> KEAIVFSQKTTIDQLHNSLNAASKTGNSNEVLQDPHIGDMYGSVTPLRPQVTRMLGKYAKEKEDMLSLRQVLANAERSYNQLMDRAAN;> VDLSDEEKDSIYMFASLVEKMKSRPLNEILEDSKLQNLAQRVFASKARLNYALNDKAQKYNTLIEMNGKISEIMNIYDRLLEQQLQSINL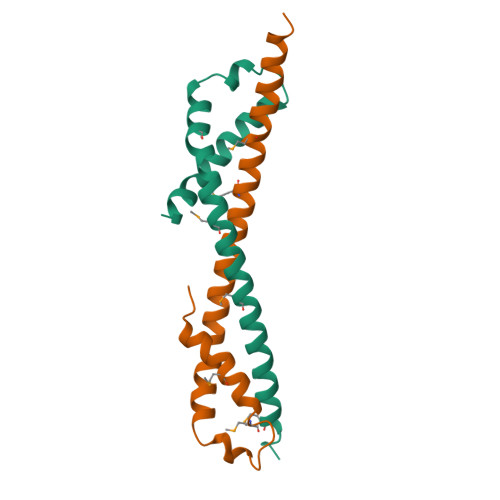S3-[5-[(4~{a}~{R},8~{a}~{S})-3-cycloheptyl-4-oxidanylidene-4~{a},5,8,8~{a}-tetrahydrophthalazin-1-yl]-2-methoxy-phenyl]-~{N}-(furan-2-ylmethyl)prop-2-ynamide 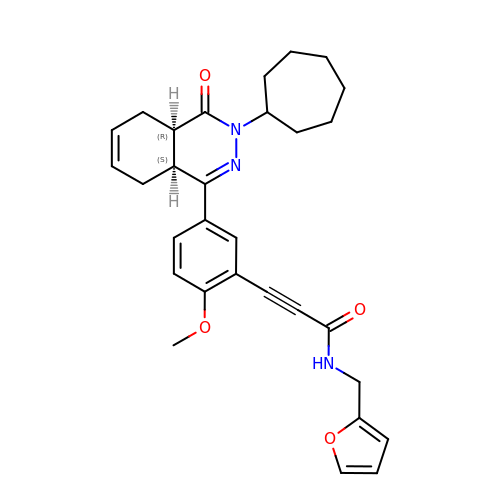| C30 H33 N3 O4 | LKXRSFQDUFXVGE-IZZNHLLZSA-N> MTAPSCAFPVQFRQPSVSGLSQI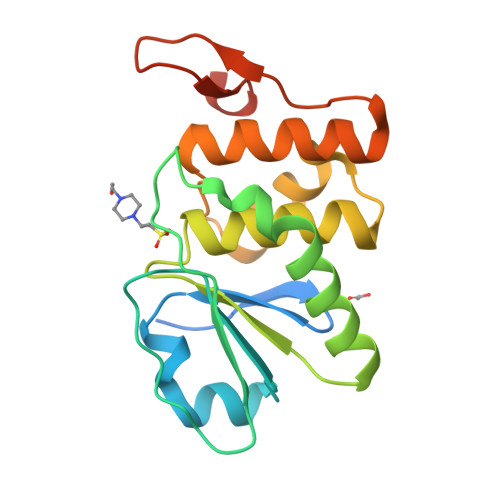TKSLYISNGVAANNKLMLSSNQITMVINVSVEVVNTLYEDIQYMQVPVADSPNSRLCDFFDPIADHIHSVEMKQGRTLLHCAAGVSRSAALCLAYLMKYHAMSLLDAHTWTKSCRPIIRPNSGFWEQLIHYEFQLFGKNTVHMVSSPVGMIPDIYEKEVRLMIPL5-(4-fluoranylphenoxy)pyridin-2-amine 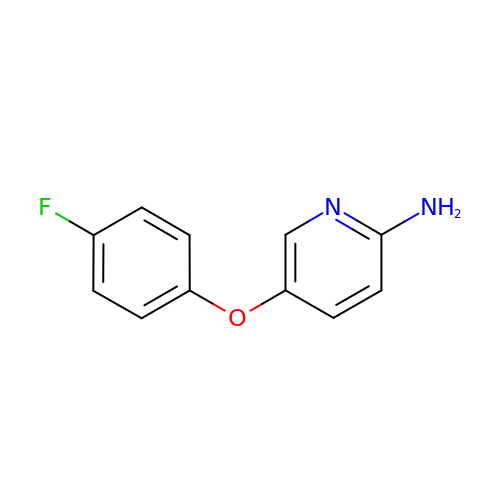| C11 H9 F N2 O | GJYQBDCLIHYVSB-UHFFFAOYSA-N Proteins containing a FIC domain catalyze AMPylation and other post-translational modifications (PTMs). Among these, Bartonella effector proteins (Beps) comprise a particularly diverse ensemble of FIC domains that subvert various host cellular functions. The FIC fold comprises eight conserved α-helices and encompasses a characteristic active site loop between helices α4 and α5 that forms most of the catalytic center and the substrate binding pocket. Additionally, FIC domains generally contain a β-hairpin between helix α2 and helix α3 that is referred to as the “flap” and mediates docking of a target segment in extended conformation via β-strand augmentation.

The structures of Bhe_BepA, Bcl_Bep1, Bqu_BepC, and Btr_BepC exhibit all features defining a FIC AMP transferase as described in the first chapter and elsewhere. However, BepC proteins are special in that they have a lysine instead of a Mg2+-coordinating aspartate/glutamate in the FIC motif. Thus, BepC proteins appear to require no divalent cation for substrate binding, in contrast to all FIC AMP transferases characterized so far. For the FIC domain of BepC with its non-canonical FIC signature motif, no enzymatic activity has been found although it binds to the RhoGEF GEF-H1 and activates this signaling protein by relocalization to the plasma membrane. For BepC, despite its canonical signature motif, no catalytic activity has yet been found, but its BepFIC domain mediates protein–protein interaction with the RhoGEF GEF-H1, thereby activating RhoA signaling. Bqu_BepC FIC with ADP crystals were grown from a solution of 15% w/v PEG 3350 and 0.1 M sussinic acid. Data for Bqu_BepC FIC with ADP, Bcl_Bep1 FIC, and B11C_Bep8 FIC were collected at 100 K on a Rayonix MX-225 detector at a wavelength of 0.9786 Å on beamline 21-ID-F at the Advanced Photon Source (APS, Argonne, IL, USA). For all structures except Bqu_BepC FIC with ADP, the structure was solved by using a molecular replacement with Phaser.

> MAHHHHHHMEHNYFYKNSATLKNKHGIKNPRKLYERCAHETAREAVNFRLEPPPGKFDAAYLRTIHWCLFHKTFEWAGVTRDQPFTFEDGSTACMPAMRPKGYKVPFAVGSQIQRELKKLEQRLTAKNNLQGLSRQEFAANAAEVFTALDHAHPFRKGNGRTQRMFMEKLGQAAGYKIDFSLITKERMTYASIEAMQHNNPEPMKDLFEDITHPQKSLLLKEFISQM Lytic Polysaccharide Monooxygenases (LPMOs) are a recently discovered group of copper metalloenzymes that depolymerize recalcitrant polysaccharides like lignocellulose and chitin by oxidative cleavage of the glycosidic bonds. The His-brace is made up of the Cu metal center coordinated with the imidazole ring Nδ1 and backbone N atoms of the terminal His and the imidazole ring nitrogen Nε2 atom of a His located later in the protein sequence. In this study, the focus is on AA9 LPMOs, where a conserved His and Gln (His147 and Gln162 in LsAA9A) form the 2nd coordination sphere and a strong H-bonding network has been shown in the crystal structures. Our results reveal that the conserved His residue of the 2nd coordination sphere in AA9 LPMOs is generally singly protonated.

Three structures of AA9 from LsAA9A and Thermoascus aurantiacus (TaAA9A) were determined in this study. Three out of the six high resolution AA9A structures, two from Lentinus similis (two different data sets for the same enzyme) and one from Thermoascus aurantiacus, were determined in this study. The data for all the three structures extends to very high resolutions. His147 in LsAA9A and His164 in TaAA9A were investigated for the protonation states at Nδ1 and Nε2 atoms of the imidazole ring of the histidines. Here, the His residues (of the primary and secondary coordination spheres) undergo unrestrained refinement, while the residues in the rest of the structure undergo restrained refinement. Our results suggest that the His of the secondary co-ordination sphere is singly protonated at the Nε2 atom in most if not all structures. Computational studies on LsAA9A have also shown that the H2O2 co-substrate does not require proton transfer (and thus double protonation). A new experimental study further highlights that H2O2 is the co-substrate strictly required for LsAA9A glycosidic bond cleavage activity. Thus, at least for LsAA9A there is currently no evidence of His147 double protonation or proton transfer being necessary for the mechanism.

> HTLVWGVWVNGVDQGDGRNIYIRSPPNNNPVKNLTSPDMTCNVDNRVVPKSVPVNAGDTLTFEWYHNTRDDDIIASSHHGPIAVYIAPAASNGQGNVWVKLFEDAYNVTNSTWAVDRLITAHGQHSVVVPHVAPGDYLFRAEIIALHEADSLYSQNPIRGAQFYISCAQITINSSDDSTPLPAGVPFPGAYTDSTPGIQFNIYTTPATSYVAPPPSVWSGALGGSIAQVGDASLE>[2x]MDLLAELQWRGLVNQTTDEDGLRKLLNEERVTLYCGFDPTADSLHIGHLATILTMRRFQQAGHRPIALVGGATGLIGDPSGKKSERTLNAKETVEAWSARIKEQLGRFLDFEADGNPAKIKNNYDWIGPLDVITFLRDVGKHFSVNYMMAKESVQSRIETGISFTEFSYMMLQAYDFLRLYETEGCRLQIGGSDQWGNITAGLELIRKTKGEARAFGLTIPLVTK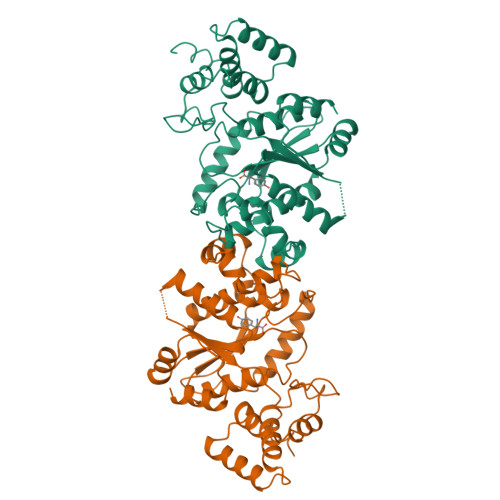ADGTKFGKTESGTIWLDKEKTSPYEFYQFWINTDDRDVIRYLKYFTFLSKEEIEALEQELREAPEKRAAQKTLAEEVTKLVHGEEALRQAIRYA>VRRGDFVRNWQLVAAVPLFQKLGPAVLVE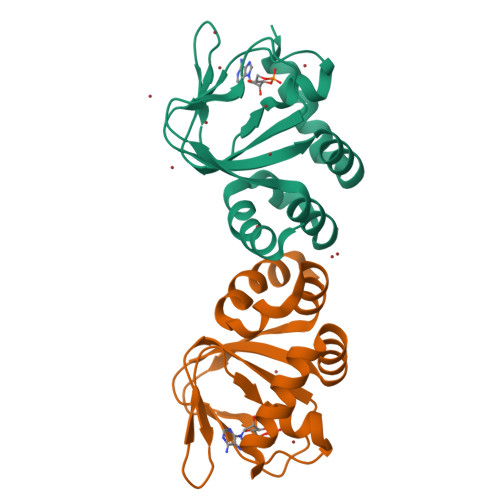IVRALRARTVPAGAVICRIGEPGDRMFFVVEGSVSVATPNPVELGPGAFFGEMALISGEPRSATVSAATTVSLLSLHSADFQMLCSSSPEIAEIFRKTALERRGAAASA[2x]> YI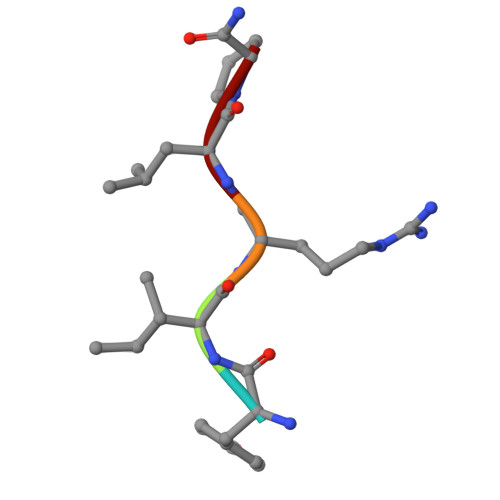RLP>KIRIGINGFGRIGRLVARVVLQRDDVELVAVNDPFITTEYMTYMFKYDSVHGQWKHNELKIKDEKTLLFGEKPVTVFGIRNPEDIPWAEAGADYVVESTGVFTDKDKAAAHLKGGAKKVVISAPSKDAPMFVVGVNEHEYKSDLDIVSNASCTTNCLAPLAKVINDRFGIVEGLMTTVHSITATQKTVDGPSMKDWRGGRAASFNIIPSSTGAAKAVGKVLPALNGKLTGMSFRVPTVDVSVVDLTVRLEKAATYDEIKKAIKEESEGKLKGILGYTEDDVVSTDFVGDNRSSIFDAKAGIALSDKFVKLVSWYDNEWGYSSRVVDLIVH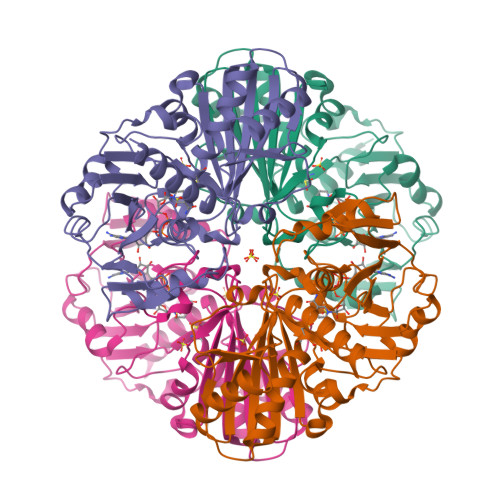MSKA[2x]> MMNDGKQQSTFLFHDYETFGTHPALDRPAQFAAIRTDSEFNVIGEPEVFYCKPADDYLPQPGAVLITGITPQEARAKGENEAAFAARIHSLFTVPKTCILGYNNVRFDDEVTRNIFYRNFYDPYAWSWQHDNSRWDLLDVMRACYALRPEGINWPENDDGLPSFRLEHLTKANGIEHSNAHDAMADVYATIAMAKLVKTRQPRLFDYLFTHRNKHKLMALIDVPQMKPLVHVSGMFGAWRGNTSWVAPLAWHPENRNAVIMVDLAGDISPLLELDSDTLRERLYTAKTDLGDNAAVPVKLVHINKCPVLAQANTLRPEDADRLGINRQHCLDNLKILRENPQVREKVVAIFAEAEPFTPSDNVDAQLYNGFFSDADRAAMKIV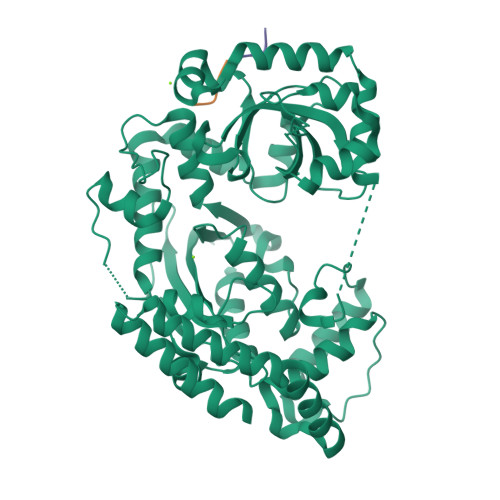LETEPRNLPALDITFVDKRIEKLLFNYRARNFPGTLDYAEQQRWLEHRRQVFTPEFLQGYADELQMLVQQYADDKEKVALLKALWQYADEIVEHHHHHH;>WMDFDDDIPF[2x]> GSHMASGAPPSVDLTSIQWRMPEWVQSMGGLRTENVLEYFSQSPFYSHKSNNEMLKMQSQFNALDLGDLNSQLKRLTGIQFVIIHERPPFLWVIQKQNRLNENEVKPLTVYFVCNENIYMAPNAYTLLATR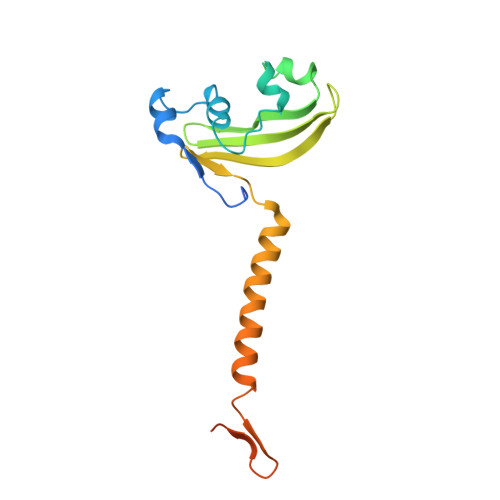MLNATYCFQKALTKIEKFPQYNPQEGYTYPKLSNDNLEVDHSNTNEPADENK> MAHHHHHHMHQVIQLKILDSRIGDTIPLPAYATDGSAGLDLRVCISEPMQVAPQQTVLLPTGIAIYIADPKLAAVILPRSGLGHKNGIVLGNLVGLIDSDYQGELKISCWNRSQEHFTVNPGDRIAQLVFIPVV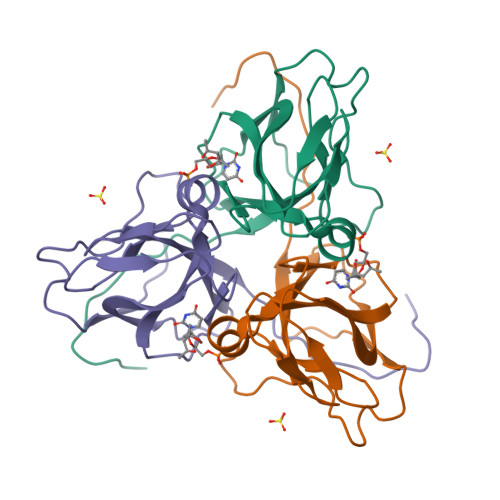QASFEVVNEFTESSRGEGGFGSSGRY>[4x]GMQTPALIIVTGHPATGKTTLSQALATGLRLPLLSKDAFKEVMFDGLGWSDREWSRRVGATA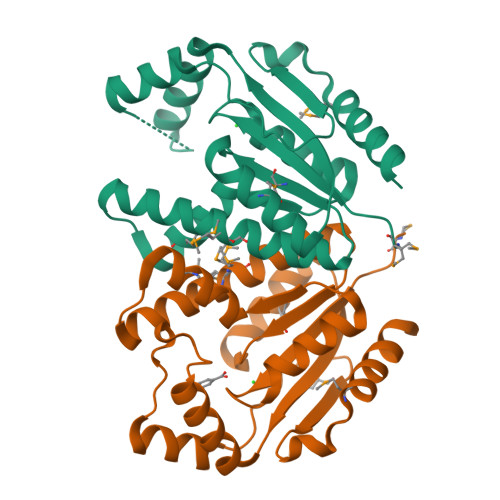IMMLYHTAATILQSGQSLIMESNFRVDLDTERMQNLHTIAPFTPIQIRCVASGDVLVERILSRIAQGARHPGHCDDRSPADLELVRSRGDIPPLPLGGPLLTVDTTFPEQIDMNAIVQWVRQHLQSGTAFL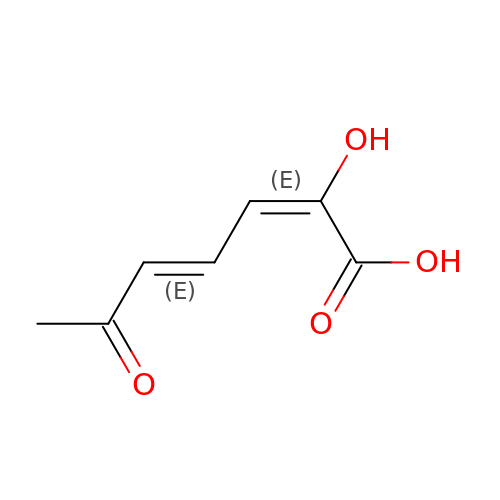(2E,4E)-2-hydroxy-6-oxohepta-2,4-dienoic acid | C7 H8 O4 | HVZGWILTESYJSP-WJPDYIDTSA-N>[4x]VVGTFKAKDLIVTPATILKEKPDPNNLVFGTVFTDHMLTVE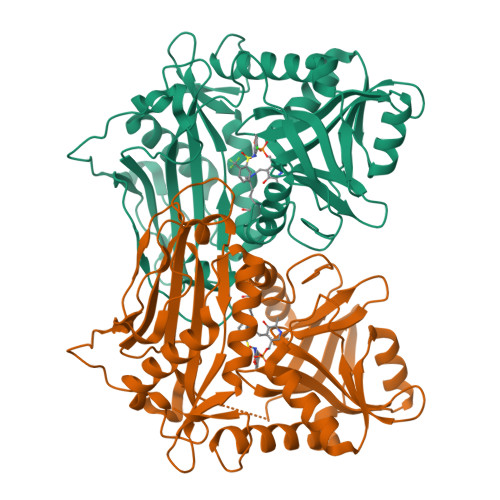WSSEFGWEKPHIKPLQNLSLHPGSSALHYAVELFEGLKAFRGVDNKIRLFQPNLNMDRMYRSAVRATLPVFDKEELLECIQQLVKLDQEWVPYSTSASLYIRPAFIGTEPSLGVKKPTKALLFVLLSPVGPYFSSGTFNPVSLWANPKYVRAWKGGTGDCKMGGNYGSSLFAQCEDVDNGCQQVLWLYGRDHQITEVGTMNLFLYWINEDGEEELATPPLDGIILPGVTRRCILDLAHQWGEFKVSERYLTMDDLTTALEGNRVREMFSSGTACVVCPVSDILYKGETIHIPTMENGPKLASRILSKLTDIQYGREESDWTIVLS> DMTQTPSSKSVPVGDTVTINCQASESVYSNNRLSWFQQKPGQPPKLLIYLVSTLASGVPSRFKGSGSGTQFTLTISDVVCDDAATYYCVGYKSSTTDGLAFGGGTEVVVKGDPVAPTVLIFPPAADQVATGTVTIVCVA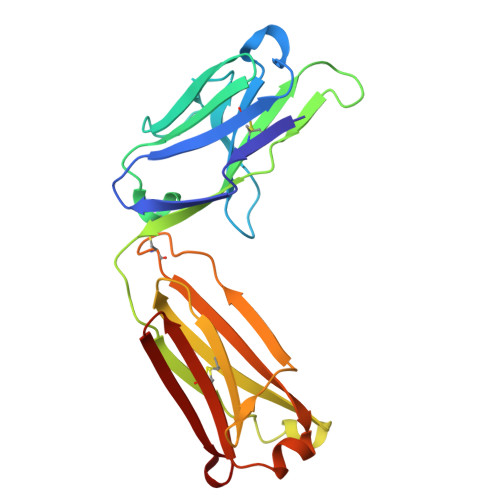NKYFPDVTVTWEVDGTTQTTGIENSKTPQNSADCTYNLSSTLTLTSTQYNSHKEYTCKVTQGTTSVVQSFNRGDC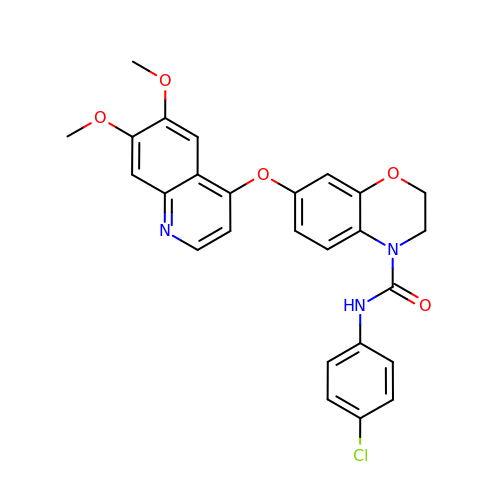N-(4-CHLOROPHENYL)-7-[(6,7-DIMETHOXYQUINOLIN-4-YL)OXY]-2,3-DIHYDRO-1,4-BENZOXAZINE-4-CARBOXAMIDE | C26 H22 Cl N3 O5 | RNHWXYKRVZUXGO-UHFFFAOYSA-N> GVDYKYKQKPKYQVRWKIIESYEGNSYTFIDPTQLPYNEKWEFPRNNLQFGKTLGAGAFGKVVEAT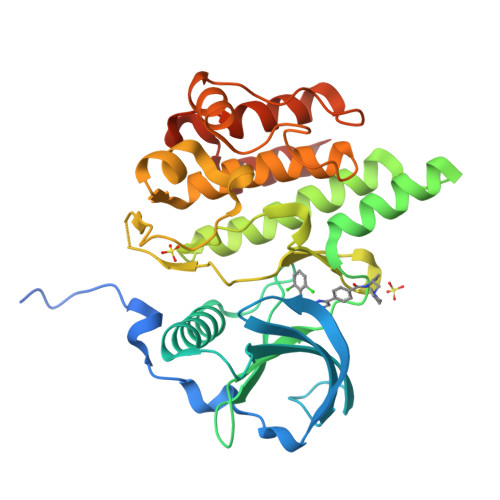AFGLGKEDAVLKVAVKMLKSTAHADEKEALMSELKIMSHLGQHENIVNLLGACTHGGPVLVITEYCCYGDLLNFLRRKAEADLDKEDGRPLELRDLLHFSSQVAQGMAFLASKNCIHRDVAARNVLLTNGHVAKIGDFGLARDIMNDSNYIVKGNARLPVKWMAPESIFDCVYTVQSDVWSYGILLWEIFSLGLNPYPGILVNSKFYKLVKDGYQMAQPAFAPKNIYSIMQACWALEPTHRPTFQQICSFLQEQAQEDRRERD>[2x]SRYIMGRTVLNESNKGLVENFSIPAELHERDGKRFASFGTTVPIHCCTPEQVAEFANKTHHYCDVFTEQVLAPLDELVYVRIDENTAE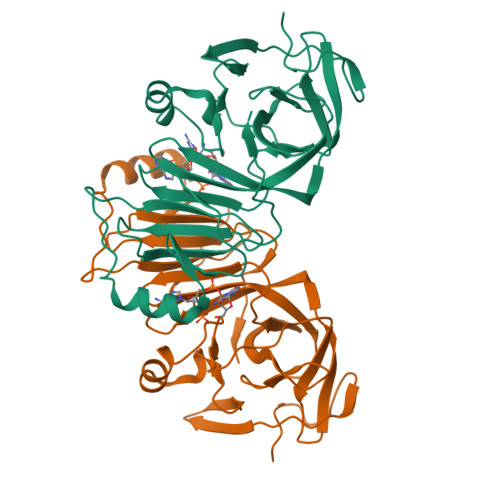KVFINRSKRILLVSSDGVLAQWRSAPTFESSNRFLAGTPIVNKDGDLVSVVTARKGNHYAVSTFEGEGGYFETSQPWKVLDPPEGAAVYGDRWFPSREEVRAYTLSLPGAAVSAGSPPAPVLHRGGSGRLVLADARGRQLSHHYLHGVATTDVQYL>MGASDDLTIEILTDDADYDLQRFDCGEEALNLFLTTHLVRQHRNKILRAYILCRNTPERQVLGYYTLCGSCFERAALPSKSKQKKIPYKNIPSVTLGRLAIDRSLQGQGWGATLVAHAMNVVWSASLAVGIHGLFVEALNEKAHTFFKSLGFIPLVGENENALFFPTKSIELLFTQSD[2x];>[2x]MAAEVIEQHRRVILNEESWTRVMDALSNPPSPGEKLKRAAKRLQG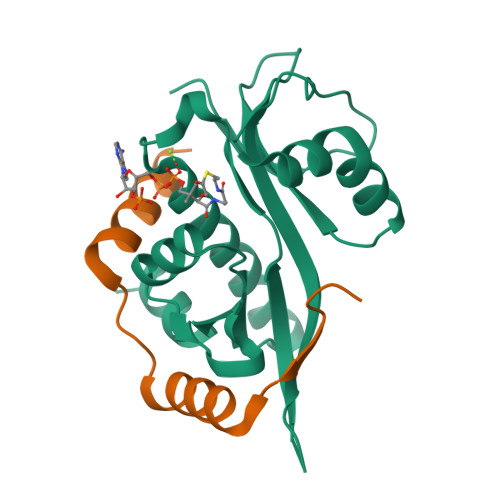M>[4x]GSHMASMYDLIIIGGGPAGLTAGIYAVRYGLDTLILERNEISGQISMADIVENYPGFPSISGLELMERFRTHAQEVGVKTTITEVLSVRSEGTKKIITTDSGDLEAKAVIIATGANPKHLGVPGEKELISKGVSYCAICDGPFFRNKIVAVVGGGNSAVTDALFLSKVAQKVYLVHRRDHLKAARVLQDRVDGTPNIELILNSHVLEIVGTREGIKKVEKIILEDVNSRETRELSTNGVFIYVGIHPNTEFVDVEKDEGGFIKTDRWMETSEKGIYAAGDCRDTPIWQLVTAVRDGAIAATAAYEYIEKIR

Thioredoxins (Trxs) participate in dithiol/disulfide exchange reactions that effect structural and functional changes in target proteins via reversible change in the redox state of selected cysteine (Cys) residues. Based on phylogenetics, protein structure, and molecular mechanism, two groups of NTRs are recognized: (i) Bacteria, plants, lower eukaryotes, and archaea contain low-molecular weight (LMW)-NTRs of about 35 kDa with a non-covalently bound flavin adenine dinucleotide (FAD) cofactor. These enzymes accept reducing equivalents from NADPH and transfer them to a redox-active disulfide motif (CxxC) that subsequently reduces Trx to its sulfhydryl form in a dithiol–disulfide exchange reaction. Thereby, according to the protein sequence comparison, MmNTR is classified as a canonical LMW-NTR.

Protein crystals of MmNTR were obtained, and the X-ray structure was solved and refined to a resolution of 2.6 Å. The X-ray structure shows that MmNTR is a homodimer, in agreement with the gel filtration data, with a structural organization that is analogous to other LMW-NTRs. Monomers consist of two Rossmann-fold domains that functionally correspond to FAD- and NADPH-binding domains. The redox motif CxxC (residues 132–136) is located on helix- α3 within the NADPH domain, with the two Cys forming a disulfide bridge in the crystal. Remarkably, no electron density of FAD or any other molecule was found at the presumed cofactor-binding pocket. The MmNTR structure thus represents the apo-form of the flavoprotein. The largest structural variations were found in a region next to the FAD-binding pocket, the so-called FAD-loop, which encompasses residues Ile37 through Pro55 (in red), that lacks a defined electron density in the apo-structure and is, therefore, omitted from the final MmNTR model. The NADPH-binding domain is positioned in an orientation with respect to the FAD-binding domain that exposes the NADPH-binding site to the bulk solvent and approaches the CxxC motif over the re-face of the isoalloxazine ring of the presumed flavin cofactor. This arrangement corresponds to the flavin-oxidizing (FO) conformation of NTRs that allows for the interaction of the disulfide bridge of the CxxC motif with the isoalloxazine ring of the flavin in a conformation competent for the reduction of the disulfide. By contrast, the FAD-binding domains slide up to the dimer interface of MmNTR with the consequent loss of α-helix contacts. Subsequently, the two domains in MmNTR are differently positioned each to the other with respect to canonical NTRs. This modification is likely a consequence of the loss of FAD, which results in the structural destabilization of the region comprising residues 36 to 68 that disrupts the dimer interface.> MRGSHHHHHHIAESKLDQILSSGELKVGTTGDWDPMAMKDPATNKYKGFDIDVMQELAKDMGVKITFVPTEWKTIVSGITAGRYDISTSVTKTPKRAEVAGFTDSYYKYGTVPLVLKKNLKKYSTWKSLNNKDVTIATTLGTSQEEKAKEFFPLSKLQSVESPARDFQEVLAGRADGNITSSTEANKLVVKYPQLAIVPDGEKNPAFLAMMVSKNDQVWNDYVNEWIKSKKSSGFFNKLLA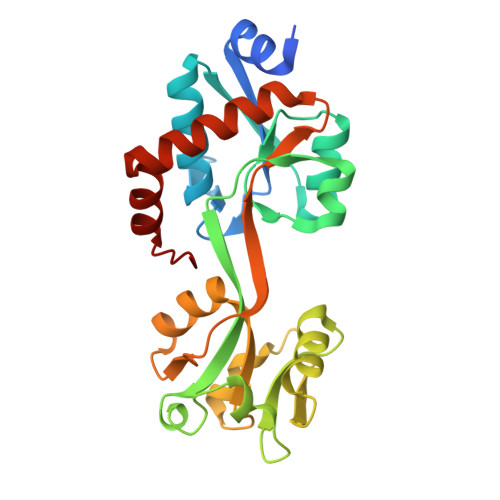KYNLKSLL>[4x]MVDFKMTKEGLVLLIKDYQNLEEVLNAISARITQMGGFFAKGDRISLMIENHNKHSQDIP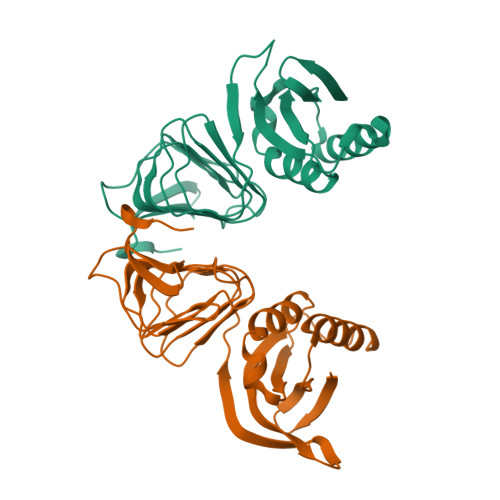RIVSHLRNLGLEVSQILVGSTVEGKENDLKVQSRTTVESTGKVIKRNIRSGQTVVHSGDVIVFGNVNKGAEILAGGSVVVFGKAQGNIRAGLNEGGQAVVAALDLQTSLIQIAGFITHSKGEENVPSIAHVKGNRIVIEPFDKVSFERSE>[2x]GSHMNLFVALYDFVAS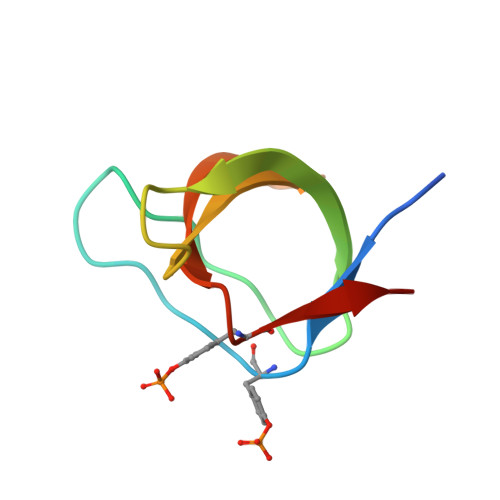GDNTLSITKGEKLRVLGYNHNGEWCEAQTKNGQGWVPSNYITPVN2,2-dimethyl-3-dehydroquinic 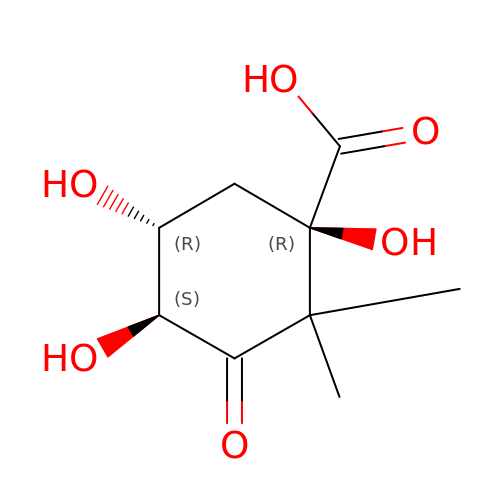acid | C9 H14 O6 | FWOMLGVRVSLROK-YZNMAWMESA-N> MATGTWNEKERKEIPGFYNRFKTQAEKSTNTGLKGRLAMPIRANWGDVGKVVTIKNDLRQLKNLFGDDMNYSAFKLGKLALLGNVKELLLYRLVDGNQKKGTLTLKDTTENSAKDVIKLETKYPTARNFN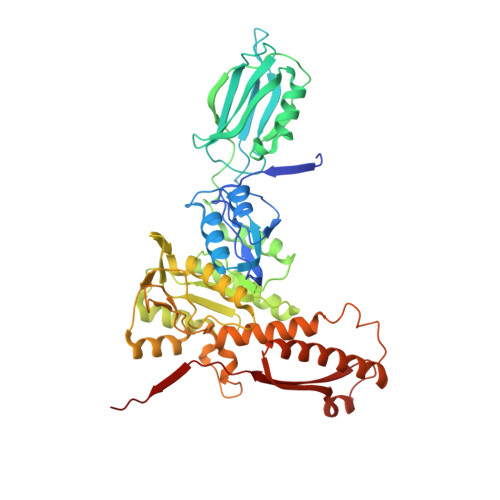VTIKSNLVDSDKKDFIFFENTKQLFSSSIKGTIDEIVLEINSNLDNEYVIATKVADSDTILANVVNQALEGGNDGCTSITNESYLKALEEFERYSFDSFVLDGVADEALQETTKAWVAKNKELGKDILLFLGGKTEDNIKQINDKSKSFNDENIVNVGSSAYYENIKYTPSEVAVYIAALSVSKGITGSICNAKTIFEEVEPRLSQSEVKECLKSGTLVLDFDDGDVIIVDDVNTFKKYVDDKNEAMGYISNIMFINTINKDTSLKRKEFVGKIFNDATGQTTVICALKKYFEELMSQGIISEFNVDIDTELQATAKADEFYWKWDAVKVDVMKKIYGTGYLG>METRRIRKVLVANRGEIAIRVFRACTELGIRTVAIYSKEDVGSYHRYKADEAYLVGEGKKPIEAYLDIEGIIEIAKAHDVDAIHPGYGFLSENIQFAKRCREEGIIFIGPNENHLDMFGDKVKARHAAVNAGIPVIPGSDGPVDGLEDVVAFAEAHGYPIIIKAALGGGGRGMRIVRSKSEVKEAFERAKSEAKAAFGSDEVYVEKLIENPKHIEVQILGDYEGNIVHLYERDCSVQRRHQKVVEVAPSVSLSDELRQRICEAAVQLMRSVGYVNAGTVEFLVSGDEFYFIEVNPRIQVEHTITEMITGIDIVQSQILIADGCSLHSHEVGIPKQEDIRINGYAIQSRVTTEDPLNNFMPDTGKIMAYRSGGGFGVRLDAGNGFQGAVITPYYDS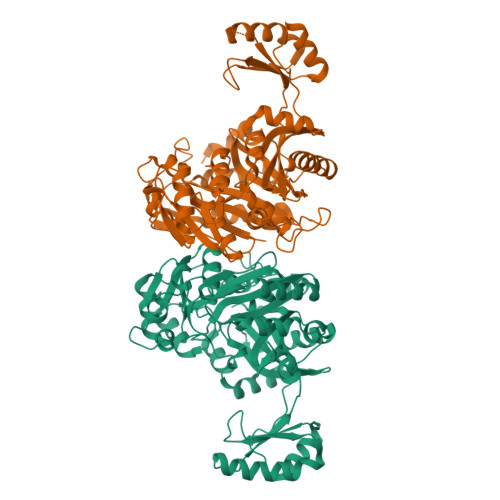LLVKLSTWALTFEQAARKMLRNLREFRIRGIKTNIPFLENVVQHPKFLSGEYDTSFIDTTPELFVF[2x]> LDRKLLTLEDKELGSGNFGTVKKGYYQMKKVVKTVAVKILKNEANDPALKDELLAEANVMQQLDNPYIVRMIGICEAESWMLVMEMAE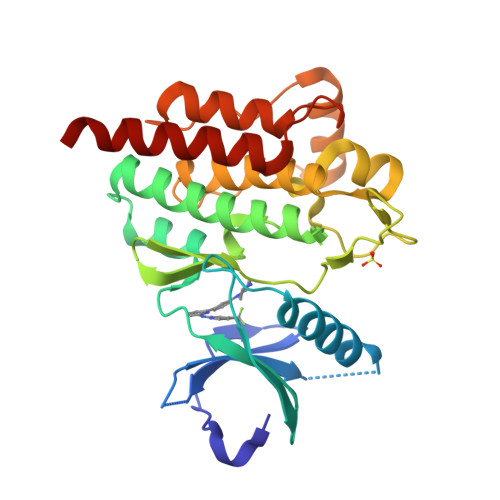LGPLNKYLQQNRHVKDKNIIELVHQVSMGMKYLEESNFVHRDLAARNVLLVTQHYAKISDFGLSKALRADENYYKAQTHGKWPVKWYAPECINYYKFSSKSDVWSFGVLMWEAFSYGQKPYRGMKGSEVTAMLEKGERMGCPAGCPREMYDLMNLCWTYDVENRPGFAAVELRLRNYYYDVVNEG> MTQAKAKHADVPVNLYRPNAPFIGKVISNEPLVKEGGIGIVQHIKFDLTGGNLKYIEGQSIGIIPPGVDKNGKPERLRLYSIASTRHGDDVDDKTISLCVRQLEYKHPESGETVYGVCSTYLTHIEPGSEVKITGPVGKEMLLPDDPEANVIMLATGTGIAPMRTYLWRMFKDAERAANPEYQFKGFS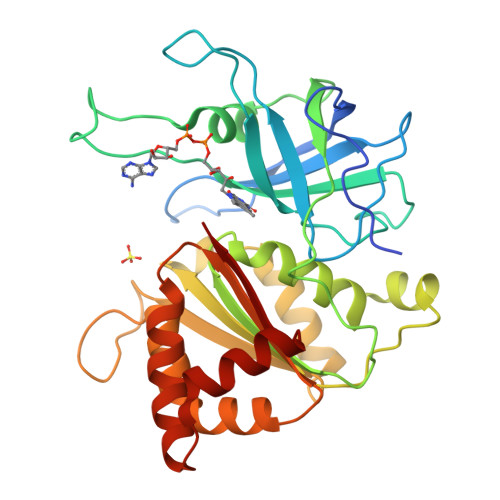WLVFGVPTTPNILYKEELEEIQQKYPDNFRLTYAISREQKNPQGGRMYIQDRVAEHADQLWQLIKNQKTHTYICGLRGMEEGIDAALSAAAAKEGVTWSDYQKDLKKAGRWHVETY Two paired rice NLR immune receptors are known that contain an integrated heavy metal-associated (HMA) domain, Pik-1/Pik-2 and RGA5/RGA4. M. oryzae secretes a large repertoire of effector proteins, and many of these, including the structurally characterized AVR–Pizt, AVR–Pia, AVR–Pik, AVR1–CO39, and AVR–Pib, share a conserved structure comprising a six-stranded β-sandwich known as the MAX (Magnaporthe Avrs and ToxB-like) fold. Direct interaction between the Pik–HMA domain and AVR–Pik is required for triggering an immune response to the effector. Here, we reveal that Pikp is able to trigger partial disease resistance to the “mis-matched” effector AVR–Pia in rice and elicits a weak cell death response in Nicotiana benthamiana.

To visualize the interface formed between Pikp–HMA and AVR–Pia, and compare it to that with AVR–Pik, we purified the complex between these proteins and determined the structure to 1.9 Å resolution using X-ray crystallography. Pikp–HMA comprises two adjacent α-helices opposite a four-stranded β-sheet. Previous structures of AVR–Pia were determined by NMR spectroscopy, and the crystal structure determined here is very similar (0.92 Å over 65 aligned residues), comprising the six-stranded β-sandwich characteristic of MAX effectors. As observed previously, a disulfide bond is formed between residues Cys-25 and Cys-66. Whereas Pikp–HMA binds AVR–PikD opposite the face of its β-sheet, it binds AVR–Pia adjacent to α-1 and β-2. Another striking feature is that whereas Pikp–HMA is a dimer in the structure with AVR–PikD, it is a monomer with AVR–Pia. The interface formed between Pikp–HMA and AVR–Pia covers an area of 460 Å2 (as calculated by PISA), approximately half of that seen between Pikp–HMA and AVR–PikD (986 Å2 (12)). Furthermore, the interface between Pikp–HMA and AVR–Pia is dominated by hydrogen bonds between the peptide backbone, with the main contributions derived from Pikp–HMAAsp-217, Pikp–HMAVal-219, AVR–PiaTyr-41, and AVR–PiaArg-43. Intriguingly, although Pikp–HMA binds AVR–Pia at a different interface to AVR–PikD, it uses the same interface that RGA5–HMA uses to bind AVR1–CO39 (29).

> GLKQKIVIKVAMEGNNCRSKAMALVASTGGVDSVALVGDLRDKIEVVGYGIDPIKLISALRKKVGDAELLQVSQA;> GPAPARFCVYYDGHLPATRVLLMYVRIGTTATITARGHEFEVEAKDQNCKVILTNGKQAPDWLAAEPY>[4x]MGHHHHHHSG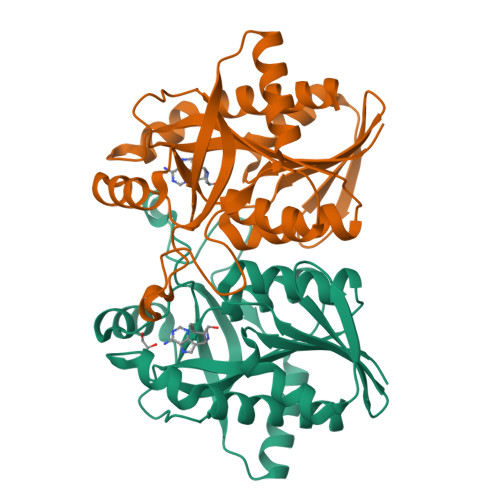MKIAILGAMSEEITPLLETLKDYTKIEHANNTYYFAKYKDHELVLAYSKIGKVNSTLSASVMIEKFGAQVLLFTGVAGAFNPELEIGDLLYATKLAQYDLDITAFGHPLGFVPGNEIFIKTDEKLNNLALEVAKELNIKLRAGIIATGDEFICDEAKKAKIREIFNADACEMEGASVALVCDALKVPCFILRAMSDKAGEKAEFDFDEFVINSAKISANFVLKMCEKL>MSQEKKVFKTEWAGRSLTIETGQLAKQANGAVLVRYGDTVVLSTATASKEPRDGDFFPLTVNYEEKMYAAGKIPGGFKKREGRPGDDATLTARLIDRPIRPLFPKGYKHDVQIMNMVLSADPDCSP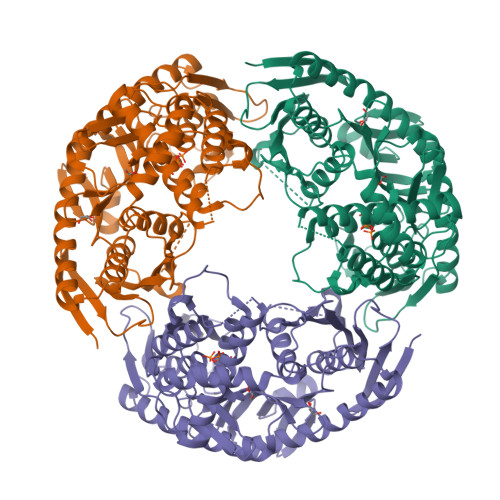QMAAMIGSSMALSVSDIPFQGPIAGVNVGYIDGKYIINPTVEEKEVSRLDLEVAGHKDAVNMVEAGASEITEQEMLEAIFFGHEEIQRLVDFQQQIVDHIQPVKQEFIPAERDEALVERVKSLTEEKGLKETVLTFDKQQRDENLDNLKEEIVNEFIDEEDPENELLIKEVYAILNELVKEEVRRLIADEKIRPDGRKPDEIRPLDSEVGILPRTHGSGLFTRGQTQALSVLTLGALGDYQLIDGLGPEEEKRFMHHYNFPNFSVGETGPVRAPGRREIGHGALGERALKYIIPDTADFPYTIRIVSEVLESNGSSSQASICGSTLALMDAGVPIKAPVAGIAMGLVTREDSYTILTDIQGMEDALGDMDFKVAGTKEGITAIQMDIKIDGLTREIIEEALEQARRGRLEIMNHMLQTIDQPRTELSHHHHHH[6x]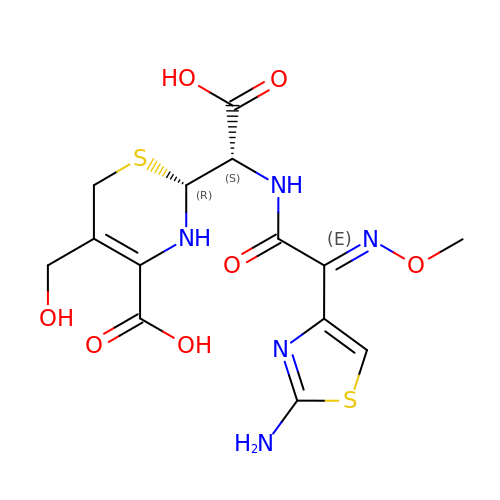(2R)-2-[(S)-{[(2E)-2-(2-amino-1,3-thiazol-4-yl)-2-(methoxyimino)acetyl]amino}(carboxy)methyl]-5-(hydroxymethyl)-3,6-dihydro-2H-1,3-thiazine-4-carboxylic acid | C14 H17 N5 O7 S2 | FGHIYDLJRRPQPG-AMEUCZBGSA-N> MKRVVITGLGIVSSIGNNQQEVLASLREGRSGITFSQELKDSGMRSHVWGNVKLDTTGLIDRKVVRFMSDASIYAFLSMEQAIADAGLSPEAYQNNPRVGLIAGSGGGSPRFQVFGADAMRGPRGLKAVGPYVVTKAMASGVSACLATPFKIHGVNYSISSASATSAHCIGNAVEQIQLGKQDIVFAGGGE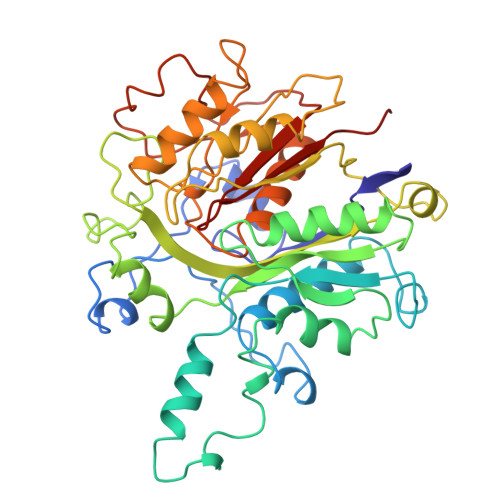ELCWEMACEFDAMGALSTKYNDTPEKASRTYDAHRDGFVIAGGGGMVVVEELEHALARGAHIYAEIVGYGATSDGADMVAPSGEGAVRCMKMAMHGVDTPIDYLNSHGTSTPVGDVKELAAIREVFGDKSPAISATKAMTGHSLGAAGVQEAIYSLLMLEHGFIAPSINIEELDEQAAGLNIVTETTDRELTTVMSNSFGFGGTNATLVMRKLKD> SPTVEECGYSDRVRSITLGNSTITTQECANVVVGYGVWPDYLKDSEATAEDQPTQPDVATCRFYTLDSVQWQKTSPGWWWKLPDALSNLGLFGQNMQYHYLGR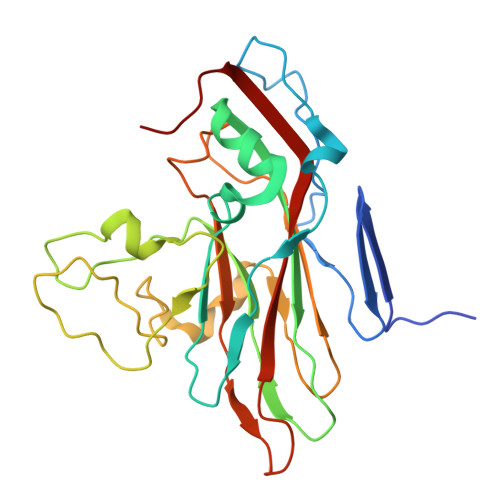TGYTIHVQCNASKFHQGCLLVVCVPEAEMGCATLNNTPSSAELLGGDTAKEFADKPVASGSNKLVQRVVYNAGMGVGVGNLTIFPHQWINLRTNNSATIVMPYTNSVPMDNMFRHNNVTLMVIPFVPLDYCPGSTTYVPITVTIAPMCAEYNGLRLAGHQ CALCIPOTRIOL | C27 H40 O3 | 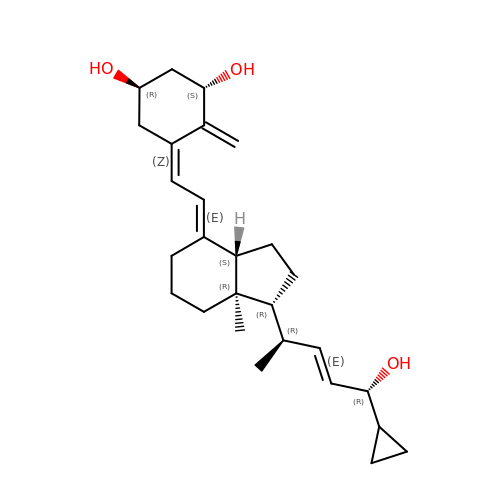LWQQLNNNIPYSNX-UROSTWAQSA-N> SMQEEDTFRELRIFLRNVTHRLAIDKRFRV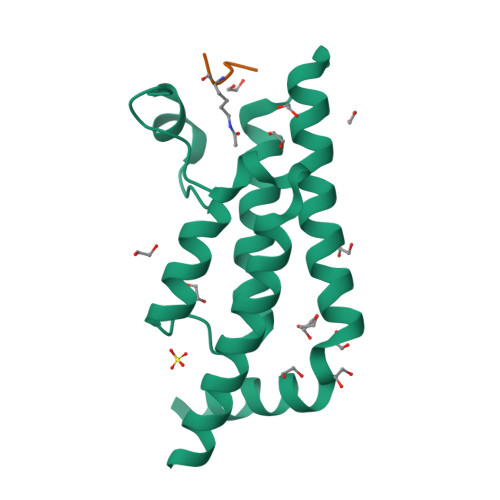FTKPVDPDEVPDYVTVIKQPMDLSSVISKIDLHKYLTVKDYLRDIDLICSNALEYNPDRDPGDRLIRHRACALRDTAYAIIKEELDEDFEQLCEEIQESR;> GLGKGGAY>MACGLVASNLNLKPGECLRVRGEVAPDAKSFVLNLGKDSNNLCLHFNPRFNAHGDANTIVCNSKDGGAWGTEQREAVFPFQPGSVAEVCITFDQANLTVKLPDGYEFKFPN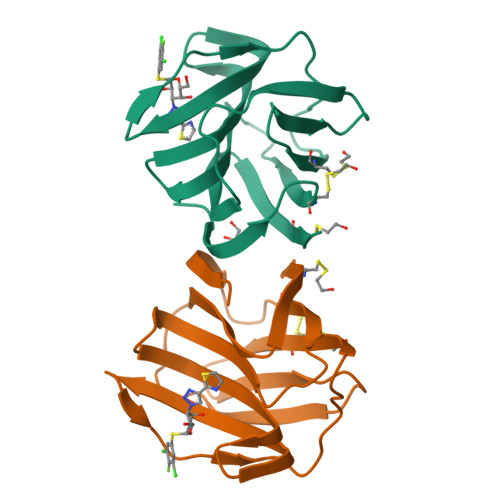RLNLEAINYMAADGDFKIKCVAFD[2x]>[3x]AHAPGTDQMFYVGTMDGWYLDTKLNSVAIGAHWSCFIVLTITTFYLGYESWTSR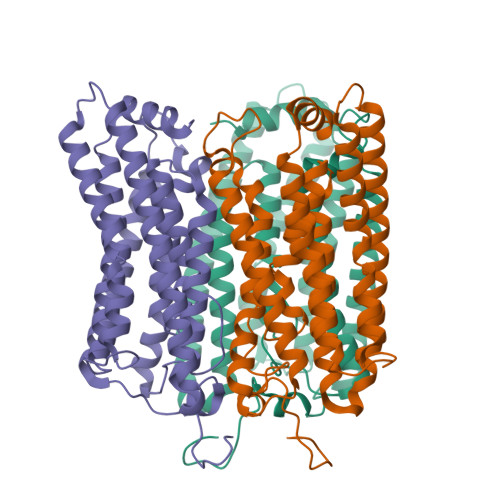GPSKRTSFYAGYQEEQNLALFVNFFAMLSYFGKIVADTLGHNFGDVGPFIIGFGNYRYADYMLTCPMLVYDLLYQLRAPYRVSCSAIIFAILMSGVLAEFYAEGDPRLRNGAYAWYGFGCFWFIFAYSIVMSIVAKQYSRLAQLAQDTGAEHSLHVLKFAVFTFSMLWILFPLVWAICPRGFGWIDDNWTEVAHCVCDIVAKSCYGFALARFRKTYDEELFRLLEQLGHDEDEFQKLELDMRLSSNGERLRRLSLNSLEVLFQ> MPLPSPNLDDRRFQQFVDDAKRYIQQRAPEWTDHNVSDPGVTLVETVAHMADQIVYRLNRVPDKNHLAFLDLVGITLFPPSAARTDVTFWLSAPQEDAILVPVGTEVATLRTERDEAVVFATEQDLRIVPCTMGRLVTQVSGEAVSDRTTDLAESKDVLCFAEAPNPGDCMLIGLSAAVPDCALALELDSRVDGVGVDPRQPPLVWEAWTEDGWQSCEVDRDGTGGLNRPGDVVLHIPGGHVLSRNGGHEAGWIRCRVTEPLSGQPFYTTSPTIRSAEAYTIGGTTGSIHAETVLDEPLGESTGLPGQRLRLEHAPVVAGEPSVLLQTAADDGWQDWQVVPHFSGSHPDDHHITVDATTGEIAFGPAVREADGTLRQYGAVPPKGAVIRARRYRTGGGRAGNVARGAVQVLRTSIPYVSEVVNREAALGGVDGETIEEAKLRAPITLRAQERAVTLRDYEELARRAAPETARITCLEGAENEYGAHAVRVLVVPQAVPDPGGRLRFEQLVPGDALLNRITRHLDERRLIGTRLAVGPPYYQGVTVVATVHAFRDVDADRVR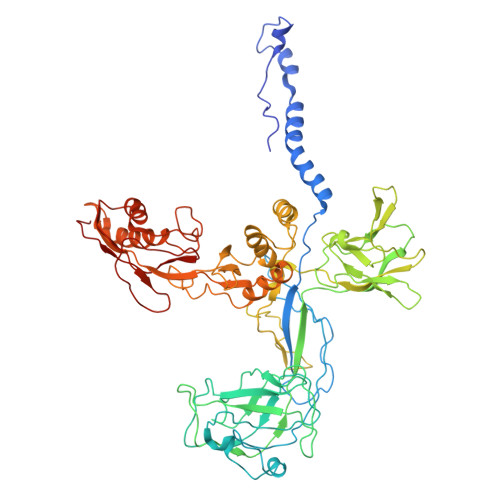RQTHDALYRHLDPLTGGSDGKGWPFGRPVQTGELFAVLQRVPGVELVDEVVLHPADPLTGKRGDPTNRIDLDAPALVFSYDHRVRVIGDSA>[4x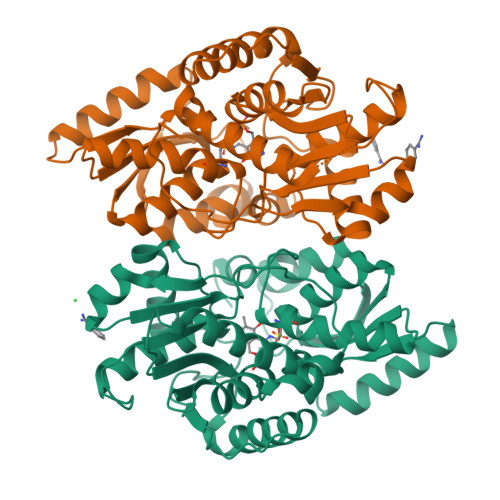]MRGSHHHHHHGMASMPLHHLTRFPRLEFIGAPTPLEYLPRLSDYLGREIYIKRDDVTPIAMGGNKLRKLEFLVADALREGADTLITAGAIQSNHVRQTAAVAAKLGLHCVALLENPIGTTAENYLTNGNRLLLDLFNTQIEMCDALTDPDAQLQTLATRIEAQGFRPYVIPVGGSSALGAMGYVESALEIAQQCEEVVGLSSVVVASGSAGTHAGLAVGLEHLMPDVELIGVTVSRSVAEQKPKVIALQQAIAGQLALTATADIHLWDDYFAPGYGVPNDAGMEAVKLLASLEGVLLDPVYTGKAMAGLIDGISQKRFNDDGPILFIHTGGAPALFAYHPHV> HHHHHHSGLVPRGSHMTAQTVTGAVAAAQLGATLPHEHVIFGYPGYAGDVTLGPFDHAAALASCTETARALLARGIQTVVDATPNDCGRNPAFLREVSEATGLQILCATGFLYEGATTYFKFRASLGDAESE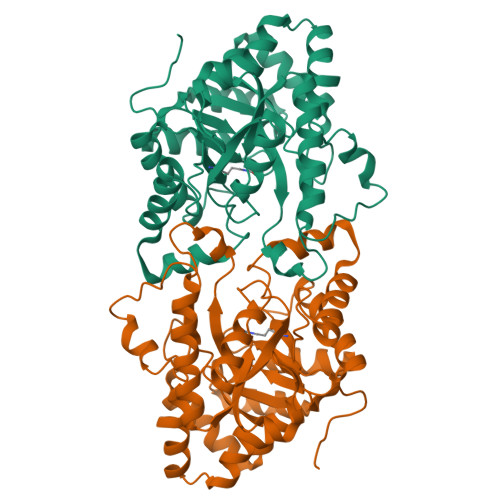IYEMMRTEVTEGIAGTGIRAGVIKLASSRDAITPYEQLFFRAAARVQRETGVPIITHTQEGQQGPQQAELLTSLGADPARIMIGHMDGNTDPAYHRETLRHGVSIAFDRIGLQGMVGTPTDAERLSVLTTLLGEGYADRLLLSHDSIWHWLGRPPAIPEAALPAVKDWHPLHISDDILPDLRRRGITEEQVGQMTVGNPARLFG> MADNEKLDNQRLKNFKNKGRDLETMRRQRNEVVVELRKNKRDEHLLKRRNVPHEDICEDSDIDGDYRVQNTSLEAIVQNASSDNQGIQLSAVQAARKLLSSDRNPPIDDLIKSGILPILVHCLERDDNPSLQFEAAWALTNIASGTSEQTQAVVQSNAVPLFLRLLHSPHQNVCEQAVWALGNIIGDGPQCRDYVISLGVVKPLLSFISPSIPITFLRNVTWVMVNLCRHKDPPPPMETIQEILPALCVLIHHTDVNILVDTVWALSYLTDAGNEQIQMVIDSGIVPHLVPLLSHQEVKVQTAALRAVGNIVTGT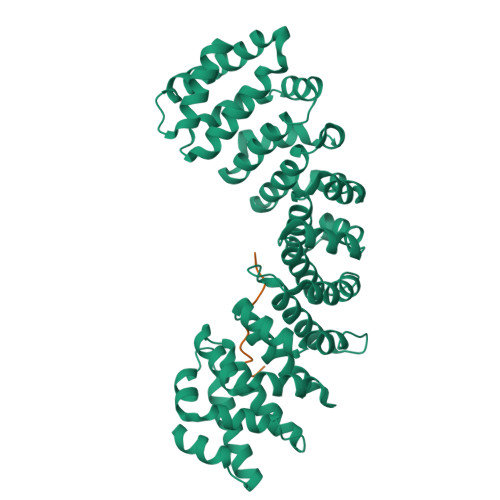DEQTQVVLNCDALSHFPALLTHPKEKINKEAVWFLSNITAGNQQQVQAVIDANLVPMIIHLLDKGDFGTQKEAAWAISNLTISGRKDQVAYLIQQNVIPPFCNLLTVKDAQVVQVVLDGLSNILKMAEDEAETIGNLIEECGGLEKIEQLQNHENEDIYKLAYEIIDQFFSSDDIDEDPSLVPEAIQGGTFGFNSSANVPTEGFQF;> DKEEVQRKRQKLMP> 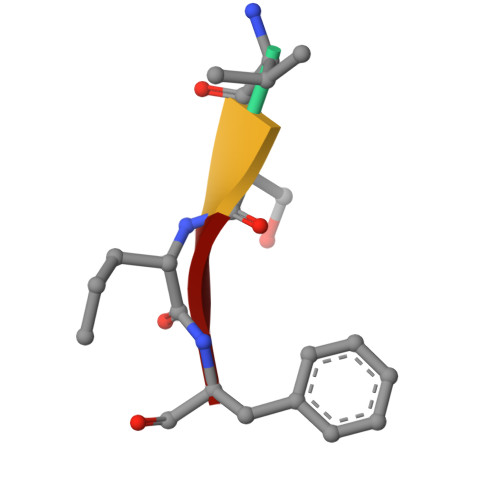VSKF[(3S,5S)-1,5-dihydroxy-2-oxopyrrolidin-3-yl]phosphonic acid | C4 H8 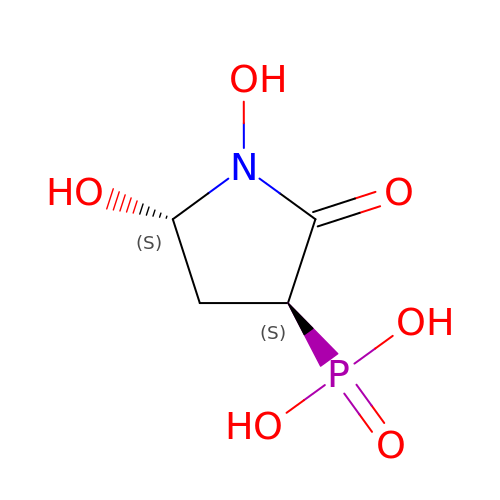N O6 P | CGWBGDOPBYWJKZ-HRFVKAFMSA-N3-METHYL-7-(5,5,8,8-TETRAMETHYL-5,6,7,8-TETRAHYDRO-NAPHTHALEN-2-YL) 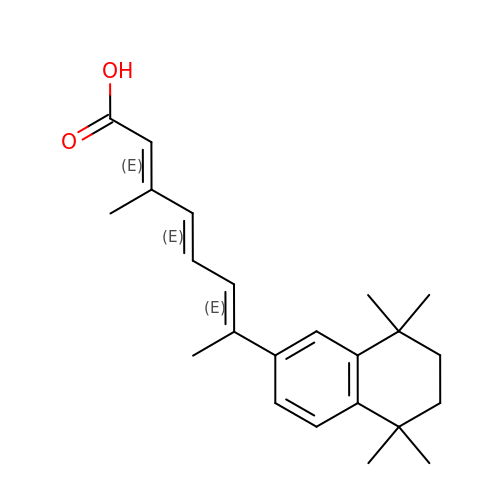-OCTA-2,4,6-TRIENOIC ACID | C23 H30 O2 | HGGVUZHIUHCATB-OOUGZNGESA-N>[6x]HMPSVIVVGGQWGDEGKGSIVAYLSLHDEPEIIARGGVGTNAGHSVVINGKKYAVRQIPTGFMQTKARLLIGAGVLVDPEVFFHELEQLKDFNVKDRVGIDY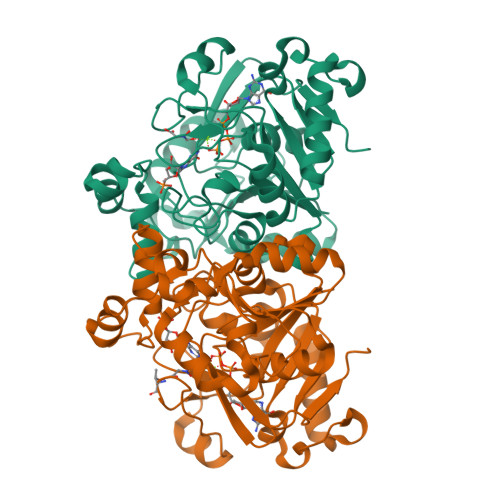RCAIIEEKHKQLDRTNGYLHGKIGTTGSGCGPANADRVMRKAKQAKDVKELEPYLTDVAQEINDALDEGSLVLVEGTQGFGLSLYYGTYPYVTSKDVTASSVAADVGIGPTRVDEVIVVFKSFPTRVGAGPFPTEMPMEEADRLGLVEYGTVTGRRRRVGWFDFEMARYSARINGATMLAVTMLDKYDKEAFGVTDYDKLPRKAKEFIEEIEERVGVPVGLIKTGPELEHIIDRRDTI Here we describe efficient routes starting from validated parallel and antiparallel peptide assemblies to design two families of α-helical barrel proteins with central channels that bind small molecules. Computational designs are seeded by the sequences and structures of defined de novo oligomeric barrel-forming peptides, and adjacent helices are connected by loop building. For targets with antiparallel helices, short loops are sufficient. However, targets with parallel helices require longer connectors; namely, an outer layer of helix–turn–helix–turn–helix motifs that are packed onto the barrels.

Our designs focused on the g-a-d-e sites of the classical coiled-coil heptad sequence repeat gabcdef, as these sites contribute most to the helix–helix interfaces. Specifically, we investigated 20 sequence combinations in which g = Ala, Gly, Leu, Met or Ser, and a and d = Ile or Leu. We solved high-resolution X-ray crystal structures of three peptides using ab initio phasing. One structure, with g-a-d-e = Ala-Leu-Ile-Ala, revealed an antiparallel hexamer consistent with its solution-phase oligomer state. However, this was a collapsed bundle, conflicting with the solution-phase binding data that suggest that this peptide can access an open α-helical barrel. Also, we have reported a parallel α-helical barrel that accesses both an open barrel and a collapsed bundle in the crystal state but still binds DPH with low micromolar affinities. Thus, it is possible that Ala-Leu-Ile-Ala and Gly-Leu-Ile-Ala can also access an open conformation in solution.

>XGALEEIAQALEEIAKALKKIAWALKKIAQGX[6x]> MEATLEQRPFPYLATEANLLTQIKESAADGLFKSFQLLLGKDAREGSVRFEALLGVYTNVVEFVKFLETALAAACVNTEFKDLRRMIDGKIQFKISMPTIAHGDGRRPNKQRQYIVMKACNKHHIGAEIELAAADIELLFAEKETPLDFTEYAGAIKTITSALQFGMDALERGLVDTVLAVKLRHAPPVFILKTLGDPVYSERGLKKAVKSDMVSMFKAHLIEHSFFLDKAELMTRGKQYVLTMLSDMLAAVCEDTVFKGVSTYTTASGQQVAGVLETTDSVMRRLMNLLGQVESAMSGPAAYASYVVRGANLVTAVSYGRAMRNFEQFMARIVDHPNALPSVEGDKAALADGHDEIQRTRIAASLVKIGDKFVAIESLQRMYNETQFPCPLNRRIQYTYFFPVGLHLPVPRYSTSVSVRGVESPAIQSTETWVVNKNNVPLCFGYQNALKSICHPRMHNPTQSAQALNQAFPDPDGGHGYGLRYEQTPNMNLFRTFHQYYMGKNVAFVPDVAQKALVTTEDLLHPTSHRLLRLEVHPFFDFFVHPCPGARGSYRATHRTMVGNIPQPLAPREFQESRGAQFDAVTNMTHVIDQLTIDVIQETAFDPAYPLFCYVIEAMIHGQEEKFVMNMPLIALVIQTYWVNSGKLAFVNSYHMVRFICTHMGNGSIPKEAHGHYRKILGELIALEQALLKLAGHETVGRTPITHLVSALLDPHLLPPFAYHDVFTDLMQKSSRQPIIKIGDQNYDNPQNRATFINLRGRMEDLVNNLVNIYQTRVNEDHDERHVLDVAPLDENDYNPVLEKLFYYVLMPVCSNGHMCGMGVDYQNVALTLTYNGPVFADVVNAQDDILLHLENGTLKDILQAGDIRPTVDMIRVLCTSFLTC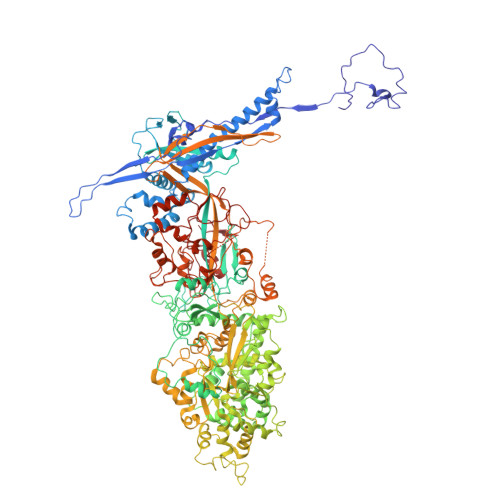PFVTQAARVITKRDPAQSFATHEYGKDVAQTVLVNGFGAFAVADRSREAAETMFYPVPFNKLYADPLVAATLHPLLANYVTRLPNQRNAVVFNVPSNLMAEYEEWHKSPVAAYAASCQATPGAISAMVSMHQKLSAPSFICQAKHRMHPGFAMTVVRTDEVLAEHILYCSRASTSMFVGLPSVVRREVRSDAVTFEITHEIASLHTALGYSSVIAPAHVAAITTDMGVHCQDLFMIFPGDAYQDRQLHDYIKMKAGVQTGPPGNRMDHVGYAAGVPRCENLPGLSHGQLATCEIIPTPVTSDVAYFQTPSNPRGRAACVVSCDAYSNESAERLLYDHSIPDPAYECRSTNNPWASQRGSLGDVLYNITFRQTALPGMYSPCRQFFHKEDIMRYNRGLYTLVNEYSARLAGAPATSTTDLQYVVVNGTDVFLDQPCHMLQEAYPTLAASHRVMLDEYMSNKQTHAPVHMGQYLIEEVAPMKRLLKLGNKVVY> GPMAWASSFDAFFKNFKRESKIISEYDITLIMTYIEENKLQKAVSVIEKVLRDIESAPLHIAVTGETGAGKSTFINTLRGVGHEEKGAAPTGAIETTMKRTPYPHPKLPNVTIWDLPGIGTTNFTPQNYLTEMKFGEYDFFIIISATRFKENDAQLAKAIAQMGMNFYFVRTKIDSDLDNEQKFKPKSFNKEEVLKNIKDYCSNHLQESLDSEPPVFLVSNVDISKYDFPKLETKLLQDLPAHKRHVFSLSLQSLTEATINYKRDSLKQKVFLEAMKAGALATIPLGGMISDILENLDETFNLYRSYFGLDDASLENIAQDLNMSVDDFKVHLRFPHL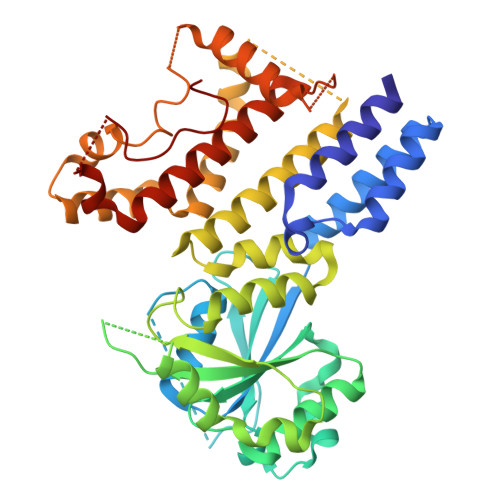FAEHNDESLEDKLFKYIKHISSVTGGPVAAVTYYRMAYYLQNLFLDTAANDAIALLNSKALFEKKVGPYISEPPEYWEA> MRGTTKPMLFLCSTAVRLNFFPLGLSAGPLNSHILLPRNNFDGRTTHGMKKIQG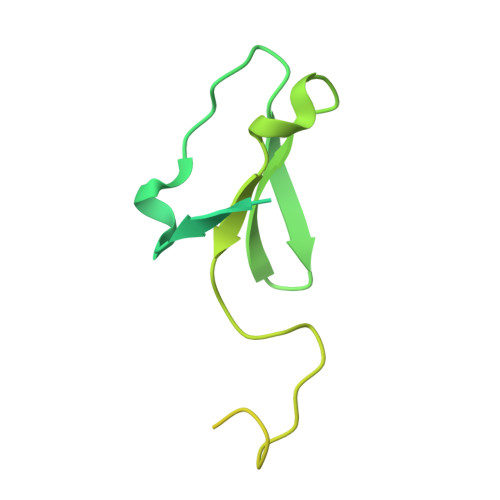QSKDPQMVMSRDELKLRCEYCRFEWIHDTLCVRCPAQPSHDQREMWLHSTWMWGKQQPYKYYKYMPAVRNPRTGMPMAREDARSMNNERRGQGLTTRTLNLEKERRGISRDVSRIGQYNTRWKTRFPFPT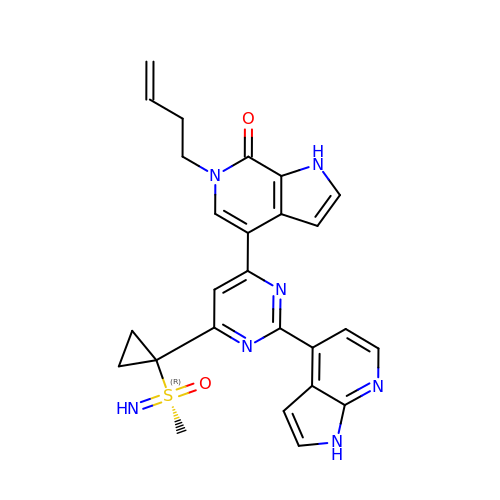6-(but-3-en-1-yl)-4-[6-{1-[(R)-S-methanesulfonimidoyl]cyclopropyl}-2-(1H-pyrrolo[2,3-b]pyridin-4-yl)pyrimidin-4-yl]-1,6-dihydro-7H-pyrrolo[2,3-c]pyridin-7-one | C26 H25 N7 O2 S | NMVFVIXUIFRHAI-PSXMRANNSA-N3-[3-(carboxymethyl)-6-(3-methoxyphenyl)-1-benzofuran-2-yl]benzoic acid | C24 H18 O6 | 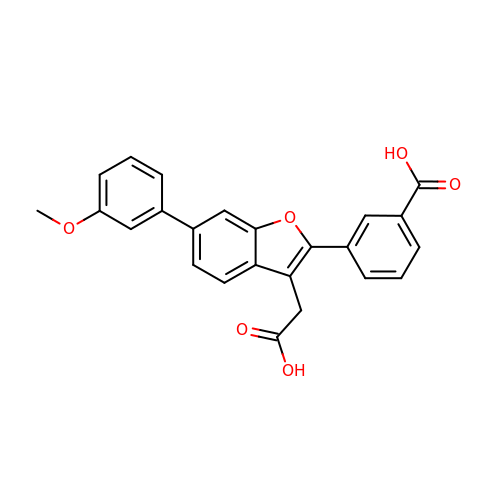OXXURMYRXBYXOG-UHFFFAOYSA-N Neprosin from the pitcher plant is a reported prolyl endopeptidase. Here, we produce recombinant neprosin and its mutants, and find that full-length neprosin is a zymogen, which is self-activated at gastric pH by the release of an all-β pro-domain via a pH-switch mechanism featuring a lysine plug. The catalytic domain is an atypical 7+8-stranded β-sandwich with an extended active-site cleft containing an unprecedented pair of catalytic glutamates. Neprosin efficiently degrades both gliadin and the 33-mer in vitro under gastric conditions and is reversibly inactivated at pH > 5.

We crystallized pro-neprosin in an orthorhombic space group and found that the polypeptide was cleaved at the physiological maturation site (P128–S129). The crystals therefore contained the zymogenic complex of the cleaved PD and the CD. We solved the structure by single-wavelength anomalous diffraction, collecting data at the lutetium LIII absorption edge wavelength from a crystal soaked in Lu-Xo440. This soaking led to significant variation in one of the crystal cell axes when compared to native crystals while keeping good diffraction of X-rays. The final refined model of the derivative complex was used to solve the native pro-neprosin structure by molecular replacement.

> METDTLLLWVLLLWVPGSTGDLMVRSIQARLANKPKGTIKTIKGDDGEVVDCVDIYKQPAFDHPLLKNHTLQMQPSSYASKVGEYNKLEQPWHKNGECPKGSIPIRRQVITGLPVVKKQFPNLKFAPPSANTNHQYAVIAYFYGNASLQGANATINIWEPNLKNPNGDFSLTQIWISAGSGSSLNTIEAGWQVYPGRTGDSQPRFFIYWTADGYTSTGCYDLTCPGFVQTNNYYAIGMALQPSVYGGQQYELNESIQRDPATGNWWLYLWGTVVGYWPASIYNSITNGADTVEWGGEIYDSSGTGGFHTTTQMGSGHFPTEGYGKASYVRDLQCVDTYGNVISPTANSFQGIAPAPNCYNYQFQQGSSELYLFYGGPGCQAIAHHHHHH> MNKKELIDRVAKKAGAKKKDVKLI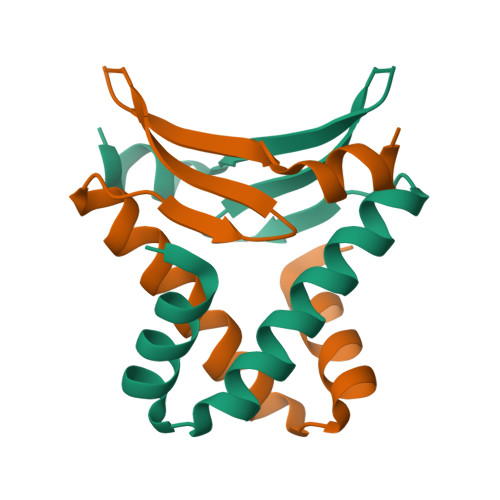LDTILETITEALAKGEKIQIVGFGSFEVRKAAARKGVNPQTRKPITIPERKVPKFKPGKALKEKVK> NLGTWRA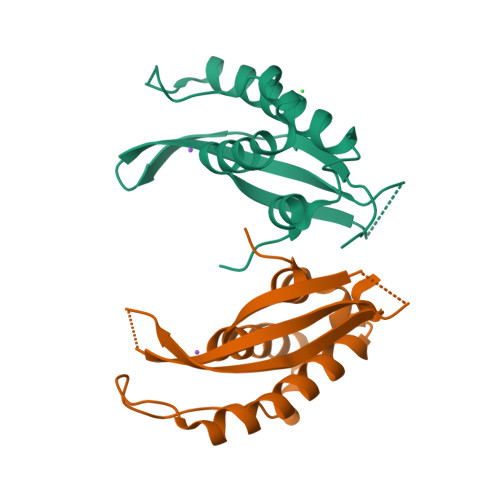VVSTAEASEENGEQMACYFVAVSLSEEDDCKNNHWTVSRKLIEFQALHRKLTECFPSLKKVQLPSLSKLPFKSIDQKFLDKSKNQLNAFLQKVLTDERMCQSEALYAFLSPSLE;> MNLGTWRAVVSTAEASEENGEQMACYFVAVSLSEEDDCKNNHWTVSRKLIEFQALHRKLTECFPSLKKVQLPSLSKLPFKSIDQKFLDKSKNQLNAFLQKVLTDERMCQSEALYAFLSPSLE Pseudomonas aeruginosa is an opportunistic pathogen that causes persistent infections in humans. Randomized transposon mutagenesis screens had indicated several genes from the diaminopimelate (DAP) biosynthetic pathway to lysine in P. aeruginosa as essential, suggesting the corresponding gene products as potential targets for new antibacterial drugs. Dihydrodipicolinate synthase (DapA) catalyzes the first committed step of the DAP pathway, the condensation of L-aspartate-semialdehyde and pyruvate to 4-hydroxy-2,3,4,5-tetrahydro-L,L-dipicolinic acid, which is non-enzymatically dehydrated to yield L-2,3-diydrodipicolinate. Tetrahydrodipicolinate N-succinyltransferase (DapD) catalyses the transfer of the succinyl moiety of succinyl-CoA to the α-amino group of tetrahydrodipicolinate, the first committed step in the succinylase branch of the DAP biosynthesis pathway present in most Gram-negative bacteria and mycobacteria.

The structure of PaDapD was determined by x-ray crystallography in its apo-form to 2.95 Å and in complex with coenzyme A and succinate to 2.3 Å resolution in the spacegroup P41212. Coenzyme A is bound in this narrow cleft formed at the interface of two adjacent subunits. CoA binds parallel to the trimer axis with the adenosine moiety positioned between the C-terminal domains of adjacent subunits. The pantetheine arm lies in the groove along the β-helix of two central domains and the β-mercaptoethylamine moiety is facing a cavity where the succinate molecule is bound. Binding of CoA to PaDapD does not induce any large conformational changes such as large scale domain re-arrangements as indicated by the r.m.s.d. value upon superposition of the subunits from the apo- and CoA complex of 0.55 Å. However CoA binding causes a disorder-order transition in the enzyme. In all structures of PaDapD that lack bound CoA, the last 15 residues including an α-helix, are not resolved in the electron density, whereas they are well defined in the PaDapD-CoA complex. The crystal structure of the complex also contains a succinate molecule bound next to the acceptor arm of the CoA in the active site cleft, most likely due to the presence of 0.4 M succinate in the crystallization buffer. Bound succinate interacts with residues from both chains that make up the active site. The position of the bound succinate corresponds well to the site of the succinyl-moiety in the ternary complexes of MtDapD and EcDapD with the co-substrate succinyl-CoA or its analogue, succinamide-CoA.

>GSHMSQSLFSLAFGVGTQNRQEAWLEVFYALPLLKPSSEIVAAVAPILGYAAGNQALTFTSQQAYQLADALKGIDAAQSALLSRLAESQKPLVATLLAEDAAPSSTAEAYLKLHLLSHRLVKPHAVNLSGIFPLLPNVAWTNIGAVDLAELAELQLEARLKGKLLEVFSVDKFPKMTDYVVPAGVRIADTARVRLGAYIGEGTTVMHEGFVNFNAGTEGPGMIEGRVSAGVFVGKGSDLGGGCSTMGTLSGGGNIVISVGEGCLIGANAGIGIPLGDRNIVEAGLYITAGTKVALLDEQNALVKVVKARDLAGQPDLLFRRNSQNGAVECKTNKTAIELNEALHAHN[3x]OXA-48 confers resistance to many carbapenem and penicillin β-lactams, but only slowly hydrolyses oxyimino-cephalosporins such as ceftazidime (CAZ). Low catalytic activity for CAZ hydrolysis has been attributed to the substrate’s bulkiness, potentially requiring sampling of alternative loop conformations to promote cephalosporin binding and hydrolysis. Here we reveal how directed evolution of a β-lactamase yielded highly epistatic activity enhancements. We describe how distinct mutations shifted the rate-limiting step from substrate binding to the chemical reaction in the β-lactamase OXA-48, thereby causing strong phenotypic epistasis.

In wtOXA-48, F72 is embedded within an aromatic pocket formed by Y144, F156, and W157, in close proximity to the active site S70. The F72L mutation disturbs this aromatic network, which probably reduces the thermostability and allows the Ω loop harbouring F156 and W157 to adapt a different conformation. Except for F72L, which reduced the Tm by 6 °C, the selected mutations barely affected the thermostability. F72L increased the IC50 by twofold, followed by a fivefold gain in IC50 through S212A. Introduction of F72L led to saturation kinetics and substantially decreased the KM to 165 ± 15 µM, suggesting an improvement in substrate binding. To estimate how the conformational dynamics changed during evolution, we performed ensemble refinements based on the crystal structures of wtOXA-48, F72L and Q5. Despite their differences in resolution, both F72L and Q5 revealed an increased flexibility primarily resulting in the Ω loop adopting various alternate conformations. Notably, F72L allows the protein to populate a different conformational ensemble, in which the space created by the loss of the phenylalanine sidechain allows the neighbouring α-helix to slide toward the centre of the protein while increasing the conformational freedom of the Ω loop. This movement is accompanied by a tightening of an H-bonding network below the Ω loop involving T71, Y144 and Q169. F72L primarily decreased the dynamical correlation between S70 and the Ω loop, which agrees with the increased flexibility and improved substrate binding conferred by F72L.

>[2x]MRVLALSAVFLVASIIGMPAVAKEWQENKSWNAHFTEHKSQGVVVLWNENKQQGFTNNLKRANQAFLPASTLKIPNSLIALDLGVVKDEHQVFKWDGQTRDIATWNRDHNLITAMKYSVVPVYQEFARQIGEARMSKMLHAFDYGNEDISGNVDSFWLDGGIRISATEQISFLRKLYHNKLHVSERSQRIVKQAMLTEANGDYIIRAKTGYSTRIEPKIGWWVGWVELDDNVWFFAMNMDMPTSDGLGLRQAITKEVLKQEKIIP> MADQAMTDQDQGAVTLYSGTAITDAKKNHPFSVKVGLAQVLRGGAIVEVSSVNQAKLAESAGACSVIVSDPVRSRGGVRRMPDPVLIKEVKRAVSVPVMARARVGHFVEAQILESLAVDYIDESEIISVADDDHFINKHNFRSPFICGCRDTGEALRRIREGAAMIRIQGDLTATGNIAETVKNVRSLMGEVRVLNNMDDDEVFTFAKKISAPYDLVAQTKQMGRVP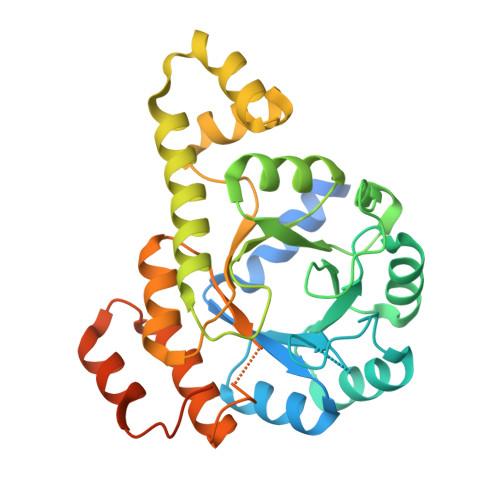VVQFASGGITTPADAALMMQLGCDGVFVGSEVFDGPDPFKKLRSIVQAVQHYNDPHVLAEMSSGLENAMESLNVRGDRIQDFGQGSVHHHHHH>MRNIRKIKVDNMKVSVYGAGNQNLYINKLNLPEKFGGEPPYGGSRMAIEFAEAGHDVVLAEPNKNIMSDDLWKKVEDAGVKVVSDDVEAAKHGEIHVLFTPFGKATFRIAKTIIEHVPENAVICNTCTVSPVVLYYSL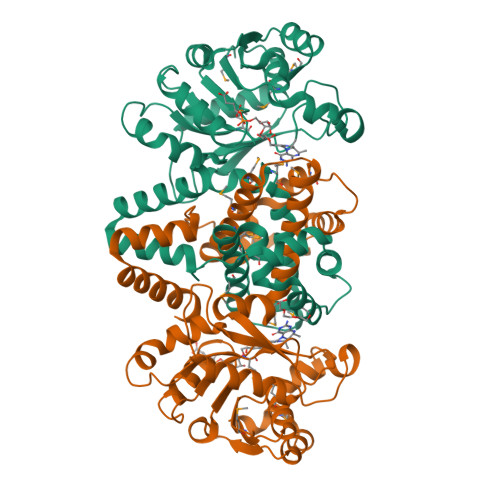EPILRTKRKDVGISSMHPAAVPGTPQHGHYVIGGKTTDGKELATEEQIKKAVELAKSAGKEAYVVPADVSSVVADMGSLVTAVALSGVLDYYTVGRKIINAPKKMIEQQVIMTLQTMASLVETSGIEGMVKALNPELLIRSASSMKLLDRQKDLDAALEILQNLDETLKAEVEKAEIKPTTLVAAQSLVKEIKTLIGGAAAEGAIKRSARKLFEHADPNSSSVDKLAAALEHHHHHH[2x]>MSTTPIDAELDLMLKRELAVPVNLVWRGLTEPELLKKWFVPKPWSISDCRVDLRPGGEFYTVMQDPEGNKFPNSGCFLEVTDEKRLIWTSALVKNY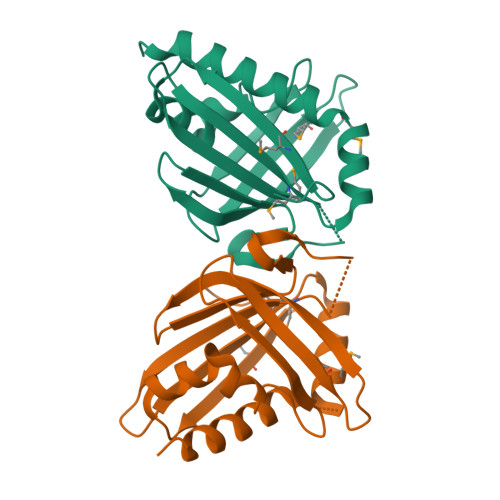RPAVPATTSDKECAHIVMTAVIELQPTSSGTRYTACAMHNTPGQRKLHEEMGFHEGWGTTITQLEELLKQEKAYLEHHHHHH[2x]>MLIIGERINGMFGDIKRAIQERDPAPVQEWARRQEEGGARALDLNVGPAVQDKVSAMEWLVEVTQEVSNLTLCLDSTNIKAIEAGLKKCKNRAMINSTNAEREKVEKLFPLAVEHGAALIGLTMNKTGIPKDSDTRLAFAMELVAAADEFGLPMEDLYIDPLILPANVAQDHAPEVLKTLQQIKMLADPAPKTVLGLSNVSQNCQNRPLINRTFLAMAMACGLDAAIADACDEALIETAATAEILLNQTVYCDSFVKMFKTR[2x];>MPLTGLEI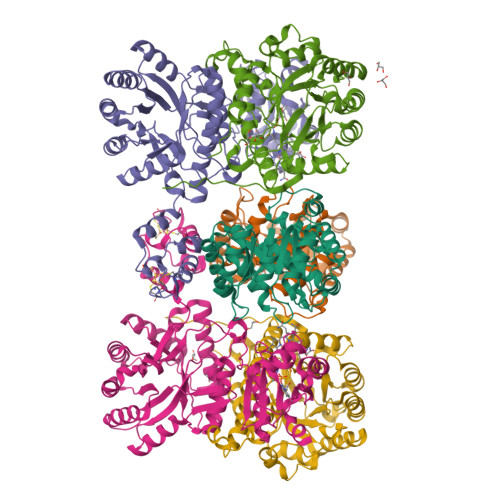YKQLPKKNCGECGTPTCLAFAMNLASGKASLDSCPYVSDAAREALDAAAAPPIAKVVLGAGPTAVEMGDETELFRHDKRFYHETAIAIQVSDNLSSEELKAKVEAINGLNFDRVGQHYTIQAIAIRHDADDPAAFKAAVASVAAATQLNLVLMADDPDVLKEALAGVADRKPLLYAATGANYEAMTALAKENNCPLAVYGNGLEELAELVDKIVALGHKQLVLDPGARETSRAIADFTQIRRLAIKKRFRSFGYPIIALTTAANPLDEVLQAVNYVTKYASLVVLRTDAKEHLLPLLSWRQNLYTDPQVPIRVEEKLNEIGAVNENSPVYVTTNFSLTYYSVEGEIESTKIPSYLLSVDTDGLSVLTAYADGKFEAEKIAAVMKKVDLDNKVKRHRIIIPGAVAVLKGKLEDLTGWEVIVGPREASGIVAFARANLAS[2x];>[2x]MAVQILRDRSRAAVQKVVLGATKDQGGTRSHTIVVGGDAALPFHHFEGEIVNRPVIGMEVQDIVPDWPDVLKDPFTDVINEPGRWAQKCVAEYGADLIYLKLDGADPEGANHSVDQCVATVKEVLQAVGVPLVVVGCGDVEKDHEVLEAVAEAAAGENLLLGNAEQENYKSLTAACMVHKHNIIARSPLDINICKQLNILINEMNLPLDHIVIDPSIGGLGYGIEYSFSIMERIRLGALQGDKMLSMPVICTVGYEAWRAKEASAPVSEYPGWGKETERGILWEAVTATALLQAGAHILLMRHPEAVARVKENIDQLMVSNAY>MVESTTTIYDVARVAGVSMATVSRVVNGNANVKEKTRQKVLEAIAELDYRPNAVARGLASKRTTTVGVILPTITSTYFAAITRGVDDIASMYKYNMILANSDNDVEKEEKVLETFLSKQVDGIVYMGSSLDEKIRTSLKNSRTPVVLVGTIDGDKEIPSVNI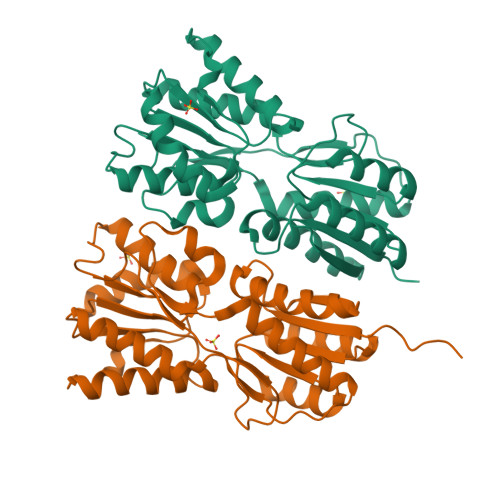DYHLAAYQSTKKLIDSGNKKIAYIMGSLKDVENTERMVGYQEALLEANIEFDENLVFEGNYSYEQGKALAERLLERGATSAVVSHDTVAVGLLSAMMDKGVKVPEDFEIISGANSPITQYTYPTLTSVNQPLYDLGAVAMRLLTKLMLKEDVEQNQLVLDHEIFSRRSTK[8x]>MTYAVAFRLERGLVFAADTRTNAGVDNIAQYKKLQLWRQPGERVFVLLSAGNLAATQAVVSLINEHLSQETDDEVTTLFTAPNMYRAARVVGDAVREARSIDGAALEASKLGFNTNFIFGGQIKGERPRLFQIYPEGNFIEATDDTPFFQIGEHKYGKPILDRVARSDMRLGEAAKLMLLSFDSTLRSNLSVGMPIDLVIYERDTFDVTREKRISADDEYFRNLSNAWSDALRQAFSKIEE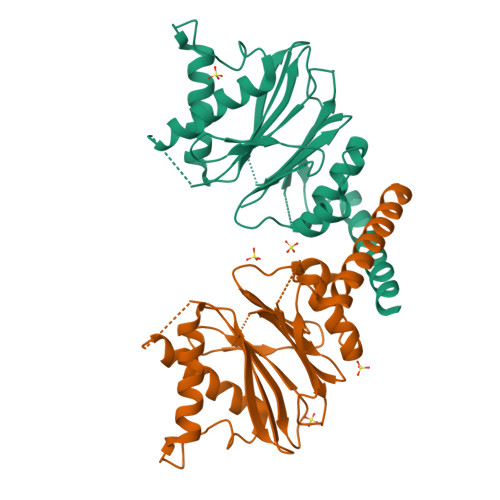FDV[2x]> MSFNSRESSLADGQPVRLYQFSRGAIRWSYNSSDRDITYQNQIFRTVPGGITDNGIICSGDPQSDQFVITAPADLDVALLYKTRSPSDAIDLVVYDMHYGDAEAAVSWVGQ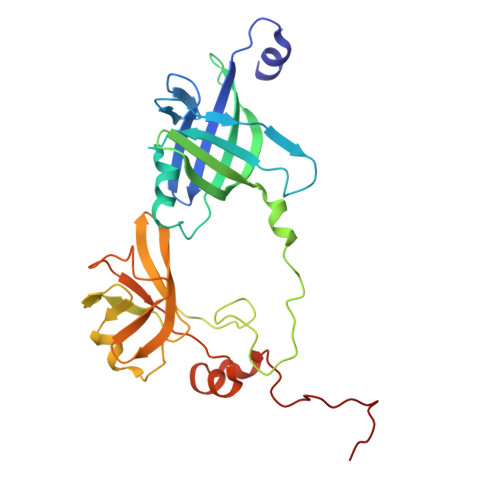IGDVDWPTVDSCRITCVSEDELMDQPGLTDTYCRTCTAIVGDHRCKVNLVPYRVTLTPQSVSAWVISSGVVAGYADGWFTGGYVEWQVDGDNYDRRFIEQHAGADLHILGGTEGIPAGGQLRVYPGCDGLAQTCDDKFSNLPNFRGFNAMQGKSPFDGDQVW To date, more than 10 MARTX effector domains have been annotated, including several domains of unknown function in Vibrio species, among which the fifth domain of a MARTX toxin from Vibrio vulnificus CMCP6 is a Ras/Rap1-specific endopeptidase (RRSP). RRSP catalyzes sequence-specific cleavage of the Switch I region of the cellular substrates Ras and Rap1 (18, 19) that are critical for a myriad of signal transduction events, including innate immune defenses. Structural and functional bioinformatics and cell biological studies revealed that RRSP belongs to the TIKI superfamily, and it is composed of an N-terminal region mediating its localization to the plasma membrane and a C-terminal region responsible for cytotoxicity. In this study, we determined the crystal structure of an RRSP from the sepsis-causing pathogen V. vulnificus CMCP6 (VvRRSP), and we demonstrated that it is a metal-independent TIKI family endopeptidase.

Deletion of N- and C-terminal flexible regions resulted in a core construct (residues 3596–4072) that produced crystals diffracting X-rays to 2.7 Å, with four VvRRSP molecules in the asymmetric unit (see under “Experimental procedures” for detailed information on structure determination and refinement). The structure of each of the four protein chains is essentially identical, except for the N-terminal α1 helix spanning residues 3596–3609. Size-exclusion chromatography revealed that VvRRSP exists as a monomer in solution; hence, the structure of chain A was considered representative of the subunit structure and was used in further analysis. The enzyme activity of VvRRSP (residues 3596–4072) was confirmed by in vitro KRas cleavage assay, demonstrating that the construct was functional and processed Ras and Rap1. The VvRRSP structure can be divided into an N-terminal lobe (N lobe, residues 3596–3722) and a C-terminal lobe (C lobe, residues 3740–4072), and the N lobe can be further subdivided into the membrane localization N1 domain (MLD), consisting of four helices (α1–α4), as characterized previously, and the N2 domain comprising three helices (α5-α7). The C lobe can also be separated into two subdomains, the C1 domain (α8–α12 and β1–β3), and the C2 domain (α13–α22 and β4–β11) that adopts a typical α + β TIKI fold. The structure of RRSP reveals that Asp-3721 on α7 forms a salt bridge with Arg-3841 on α12 that helps to maintain the structure between N2 and C1 domains. During refinement of the RRSP structure, we noticed that the electron density map around residues Arg-3988–Gln-3992 located close to the active site in the C2 domain is disordered, indicating flexibility and a potential involvement in substrate recognition. Although we did not observe any metal bound to VvRRSP during refinement of its structure, we biochemically examined whether it belongs to the TIKI metalloprotease family. Superimposition of VvRRSP molecules in the asymmetric unit reveals different conformations for the MLD fingers, indicating flexibility.

>GAMAQELKERAKVFAKPIGASYQGILDQLDLVHQAKGRDQIAASFELNKKINDYIAEHPTSGRNQALTQLKEQVTSALFIGKMQVAQAGIDAIAQTRPELAARIFMVAIEEANGKHVGLTDMMVRWANEDPYLAPKHGYKGETPSDLGFDAKYHVDLGEHYADFKQWLETSQSNGLLSKATLDESTKTVHLGYSYQELQDLTGAESVQMAFYFLKEAAKKADPISGDSAEMILLKKFADQSYLSQLDSDRMDQIEGIYRSSHETDIDAWDRRYSGTGYDELTNKLASATGVDEQLAVLLDDRKGLLIGEVHGSDVNGLRFVNEQMDALKKQGVTVIGLEHLRSDLAQPLIDRYLATGVMSSELSAMLKTKHLDVTLFENARANGMRIVALDANSSARPNVQGTEHGLMYRAGAANNIAVEVLQNLPDGEKFVAIYGKAHLQSHKGIEGFVPGITHRLDLPALKVSDSNQFTVEQDDVS[4x]> ICVNENGGCEQYCSDHTGTKRSCRCHEGYSLLADGVSCTPTVEYPCGKIPILEKRNASKPQ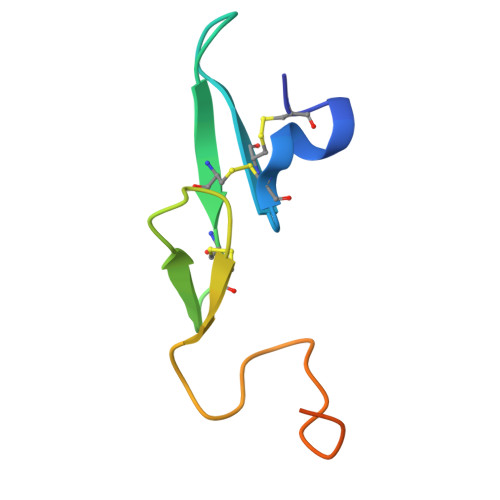GR> MAVTDLSLTNSSLMPTLNPMIQQLALAIAASWQSLPLKPYQLPEDLGYVEGRLEGEKLVIENRCYQTPQFRKMHLELAKVGKGLDILHCVMFPEPLYGLPLFGCNIVAGPGGVSAAIADLSPTQSDRQLPAAYQKSLAELGQPEFEQQRELPPWGEIFSEYCLFIRPSNVT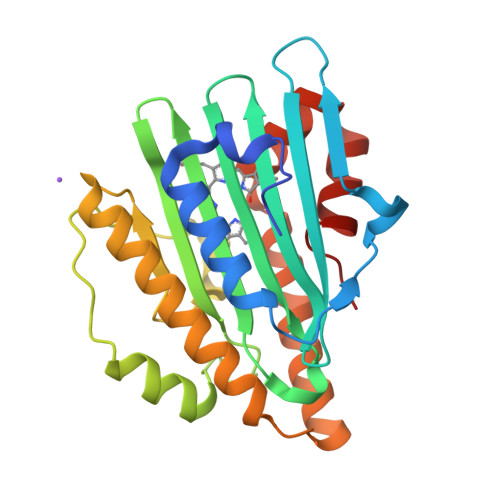EEERFVQRVVDFLQIHCHQSIVAEPLSEAQTLEHRQGQIHYCQQQQKNDKTRRVLEKAFGEAWAERYMSQVLFDVIQ>[4x]MSLKYQLRFGGEGGQGVITAGEILAEAAIKEGRQAFKASTYTSQVRGGPTKVDIIIDDKEILFPYAVEGEVDFMLSTADKGYKGFRGGV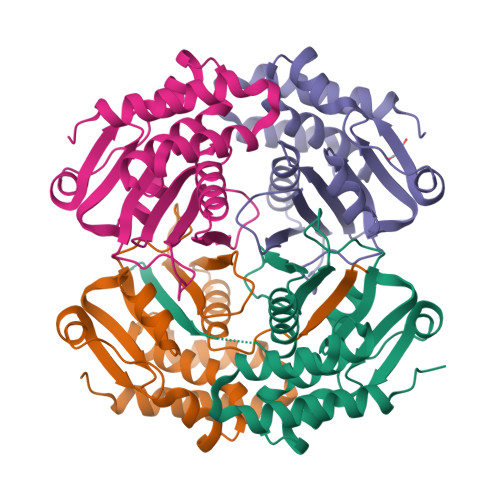KEGGIIVVEPNLVHPESEDYKKWQIFEIPIITIAKDEVGNVATQSVVALAIAAYMSKCIDLDVLKETMLHMVPAKTRDANAKAFDLGVKYATQAKPHEGHHHHHH>AEGQTNADDTLVVEASTPSLYAPQQSADPKFSRPVADTTRTMTVISEQVIKDQGATNLTDALKNVPGVGAFFAGENGNSTT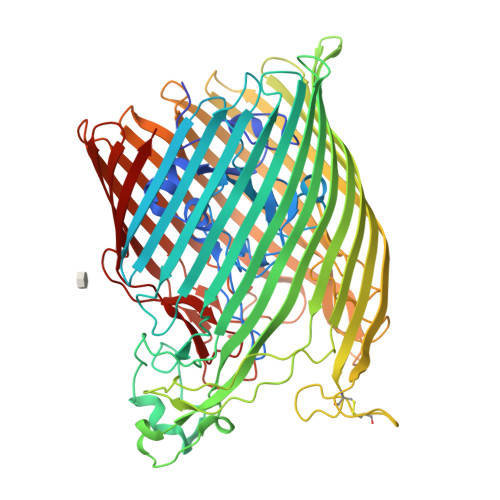GDAIYMRGADTSNSIYIDGIRDIGSVSRDTFNTEQVEVIKGPSGTDYGRSAPTGSINMISKQPRNDSGIDASASIGSAWFRRGTLDVNQVIGDTTAVRLNVMGEKTHDAGRDKVKNERYGVAPSVAFGLGTANRLYLNYLHVTQHNTPDGGIPTIGLPGYSAPSAGTAALNHSGKVDTHNFYGTDSDYDDSTTDTATMRFEHDINDNTTIRNTTRWSRVKQDYLMTAIMGGASNITQPTSDVNSWTWSRTANTKDVSNKILTNQTNLTSTFYTGSIGHDVSTGVEFTRETQTNYGVNPVTLPAVNIYHPDSSIHPGGLTRNGANANGQTDTFAIYAFDTLQITRDFELNGGIRLDNYHTEYDSATACGGSGRGAITCPTGVAKGSPVTTVDTAKSGNLMNWKAGALYHLTENGNVYINYAVSQQPPGGNNFALAQSGSGNSANRTDFKPQKANTSEIGTKWQVLDKRLLLTAALFRTDIENEVEQNDDGTYSQYGKKRVEGYEISVAGNITPAWQVIGGYTQQKATIKNGKDVAQDGSSSLPYTPEHAFTLWSQYQATDDISVGAGARYIGSMHKGSDGAVGTPAFTEGYWVADAKLGYRVNRNLDFQLNVYNLFDTDYVASINKSGYRYHPGEPRTFLLTANMHF[4x]>[2x]MAHHHHHHHRSSLTNVGNDRHAAGTDTDRARERDRRHLWHPWSSVRQPADDRPILVAGEGCRVRDVTGAGYLDAMASAMNSSCGYAHPALLEAARRQLELLPHFDLSAASHLPAGLAAERIAGLLPAGLERTFFVNSGSEATEAAVRIAHDHWTNRGEPRDRLVTFAAGYHGTTLVAQHLSGLPTNAIHGTAPFPVTRVELPLEPAALRTPEALTLLADAFERAVLDGPPPAAVMVEPLLNVGGGVVLPDGFLRALRALCDRTGALLIVDEVFCGFGRTGRMFGFQHDGVTPDLVTMSKGISGGYVPFAALTTTDEVYRSFAADPLLGGLRYGHTTGGHAVACAVALAVLDVIEERGLVGSAARLGAELLAGLAPLAEHPEVTDVRGLGLVATVECRQPESAAALVAEAKRQGVLLRQQGRAVMAIPPLVIDAAEVAELVRAVEQAVARL

Pseudouridimycin is a microbial C-nucleoside natural product that specifically inhibits bacterial RNA polymerases by binding to the active site and competing with uridine triphosphate for the nucleoside triphosphate (NTP) addition site. Conversion to pseudouridine aldehyde via alcohol oxidation by PumI (SapB in S. albus DSM 40763) and subsequent amine formation to 5′-aminopseudouridine by PumG (SapH in S. albus DSM 40763) are the likely sequential biosynthetic steps. The pyridoxal phosphate (PLP)-dependent SapH catalyzes transamination, resulting in 5′-aminopseudouridine with a preference for arginine, methionine, or phenylalanine as cosubstrates as amino group donors. The binary structure of SapH in complex with pyridoxamine-5′-phosphate and site-directed mutagenesis identified Lys289 and Trp32 as key residues for catalysis and substrate binding, respectively.

The structure of SapH was determined to a 1.55 Å resolution by X-ray crystallography in space group P212121 using molecular replacement. The asymmetric unit of the crystals contains a tightly packed dimer, and each polypeptide chain shows the fold characteristic for PLP enzymes of the fold type I, subclass II. The overall fold and the mode of dimerization seen in SapH is essentially identical to what is observed in the fold-type I aminotransferase family, for instance, in the related 7,8 diamino pelargonic acid synthase23 and 8-amino-7-oxononaoate aminotransferase24. The dimer observed in the SapH crystals most likely represents the biologically active form of the enzyme as the cofactor binding site, and the active-site pocket is built up by residues from both chains constituting the dimer. The binding site of the PLP cofactor is located close to the dimer interface, with residues from both subunits involved in cofactor–protein interactions. The bound PLP was modeled as pyridoxamine, according to the observed electron density map, and because the expected covalent link between PLP and Lys289, conserved in the protein family, is absent in the crystal structure. The aromatic ring system of PLP is sandwiched between the hydrophobic side chains of Tyr160 and Val262. The phenolic oxygen atom of PLP forms a hydrogen bond to the side chain of Asn23, and the ring nitrogen is hydrogen-bonded to the side chain of Asp260. Extending from the bound pyridoxamine 5′-phosphate (PMP) to the bulk solution, a pocket is formed that represents the active-site cavity formed by residues from both subunits and lined with hydrophobic and polar residues that might be involved in substrate binding and catalysis. At the opening of this cleft is a flexible disordered loop region (residues 35–43) that could act as a flap and close the active site once the substrate is bound.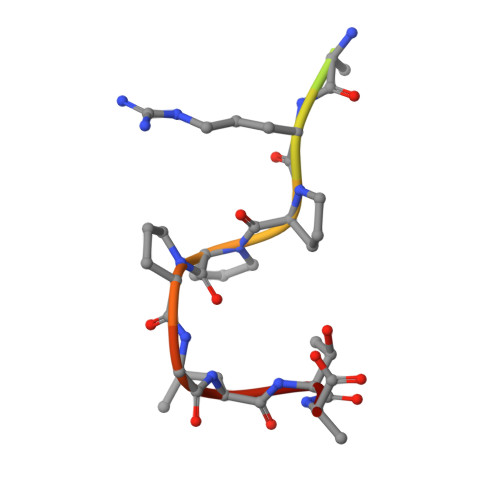> GPLGSAPTRPPPGLTN> MKLYFNGGKKKKIRAVDFVGTIAKIDGVSADDIGIITIMDNASYVE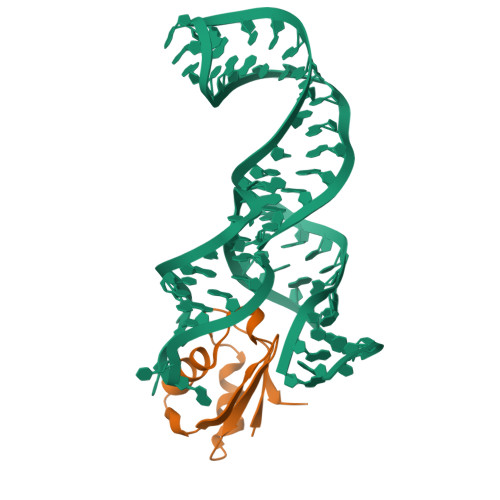ILNGKGPHVLKVMKNTTVKGKQLKVNKANK1-(7-chloranyl-4-methoxy-1~{H}-indol-5-yl)-3-[1-(phenylmethyl)piperidin-4-yl]propan-1-one 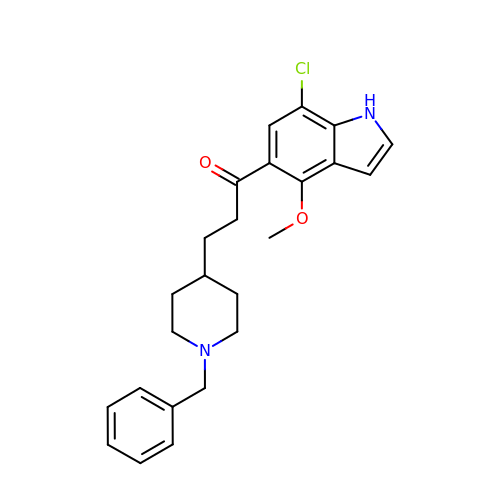| C24 H27 Cl N2 O2 | BXNNACCQTQBSOO-UHFFFAOYSA-N N-(dimethylsulfamoyl)-L-phenylalanyl-N-[(1S,2S)-2-hydroxy-4-{[(2S)-2-methylbutyl]amino}-1-(2-methylpropyl)-4-oxobutyl]-N~6~-(methylcarbamothioyl)-L-lysinamide 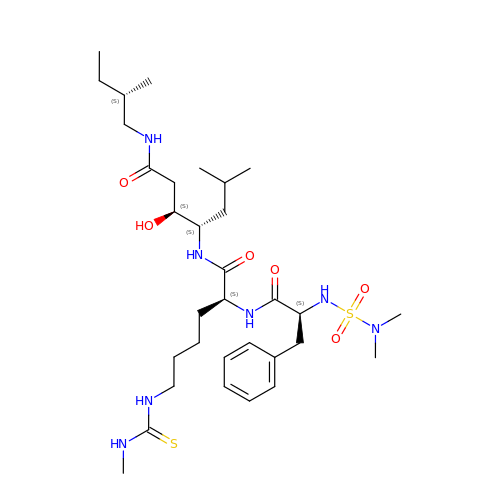| C32 H57 N7 O6 S2 | GBPRCFWBWHGSJH-BLVAWXTGSA-N>[6x]MGESERSEAFGIPRDSPLSSGDAAELEQLRREAAVLREQLENAVGSHAPTRSARDIHQLEARIDSLAARNSKLMETLKEARQQLLALREEVDRLGQPPSGYGVLLATHDDDTVDVFTSGRKMRLTCSPNIDAASLKKGQTVRLNEALTVVEAGTFEAVGEISTLREILADGHRALVVGHADEERVVWLADPLIAEDLPDGLPEALNDDTRPRKLRPGDSLLVDTKAGYAFERIPKAEVEDLVLEEVPDVSYADIGGLSRQIEQIRDAVELPFLHKELYREYSLRPPKGVLLYGPPGCGKTLIAKAVANSLAKKMAEVRGDDAHEAKSYFLNIKGPELLNKFVGETERHIRLIFQRAREKASEGTPVIVFFDEMDSIFRTRGTGVSSDVETTVVPQLLSEIDGVEGLENVIVIGASNREDMIDPAILRPGRLDVKIKIERPDAEAAQDIYSKYLTEFLPVHADDLAEFDGDRSACIKAMIEKVVDRMYAEIDDNRFLEVTYANGDKEVMYFKDFNSGAMIQNVVDRAKKNAIKSVLETGQPGLRIQHLLDSIVDEFAENEDLPNTTNPDDWARISGKKGERIVYIRTLVTGKSSSASRAIDTESNLGQYL;> GSMAQEQTKRGGGGGDDDDIAGSTAAGQERREKLTEETDDLLDEIDDVLEENAEDFVRAYVQKGGQ

Proteasomes are present in eukaryotes, archaea and Actinobacteria, including the human pathogen Mycobacterium tuberculosis, where proteasomal degradation supports persistence inside the host. In mycobacteria and other members of Actinobacteria, prokaryotic ubiquitin-like protein (Pup) serves as a degradation tag post-translationally conjugated to target proteins for their recruitment to the mycobacterial proteasome ATPase (Mpa). The bacterial 20S proteasome interacts with a ring-shaped AAA regulatory complex called the mycobacterial proteasome ATPase (Mpa) in mycobacteria or ARC (ATPase forming ring-shaped complexes) in other actinobacterial species. Here, we use single-particle cryo-electron microscopy to determine the structure of Mpa in complex with the 20S core particle at an early stage of pupylated substrate recruitment, shedding light on the mechanism of substrate translocation.

To improve the local resolution of Mpa, we performed local 3D classification and 3D refinement combined with signal subtraction of the 20S CP (see “Methods”). This approach resolved two states of Mpa at an average resolution of 3.8 Å and 3.9 Å, respectively. The two states correspond to two distinct motor conformations stalled at sequential stages of substrate translocation. A stacked pair of residues, the canonical aromatic pore loop residue F341 and the highly conserved adjacent lysine residue K340, forms a spiral-staircase that encircles the Pup N-terminal segment by engaging in unspecific interactions with its Cα backbone. Interestingly, while in state A, all six of the canonical aromatic pore loops of the ATPase domain are in close proximity to the substrate backbone with one of them (protomer 6, cyan) initially disengaged, in state B only five protomers are in close proximity to the substrate backbone and engaged in interactions with it. The loop of the penultimate protomer (protomer 6, cyan), which was at the bottom of the staircase in state A, is retracted away from the substrate in state B and has shifted upward by 25 Å to a more distal position relative to the proteasome gate. Furthermore, in state B, the five pore loops contacting the substrate are shifted downwards by 2–3 Å compared to state A, which results in a translocation of the substrate towards the open gate of the proteasome by almost one amino acid. In state B in comparison, all protomers of Mpa are resolved with ATP bound, including protomer 6 (cyan) with its pore loop now in a disengaged and retracted conformation. Nevertheless, protomer 6 still exhibits less contacts to protomer 5, and the arginine finger that it contributes to protomer 5 does not contact the nucleotide, thereby creating a fissure in the ATPase ring between these protomers.>[3x]MRTGQQYLESLRDGRQVYVGGELIDDVTTHPKTSGYAKAIAEYYDLHLDPEHQDVLTFVDDDGVRKSMHWFLPRSKADAARRRAYHEFWFRHFQGGIFTRPPAGMHVVMYAQIDDPEPWGDNAVVAGGRTISFADNIRSQWQRVTTDDVALSPMFVDVQFDRGRDDALVETPMLSIVEQNDQGIVVRGWKAMGTSLPFVNELLVGNLWRPGQTSDQTVYAIVPVNTPGLSLVCRQSNATPDADPYDHPLSTIGDELDGMAYFDDVFIPWENVQHIGNPDHAKWYPQRQFDWVHIETQIRHAVHAELIVGLALLLTNALGTNNNPIVQSQLADLVRFRETCKAFAIAAEETGFTT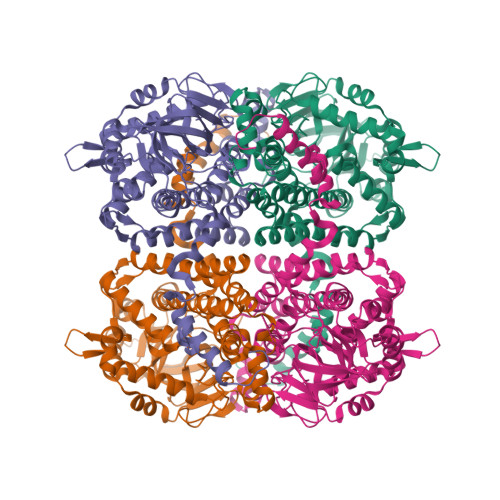AGGLFKPNNIYVDLGRAHYLENIHNAVNQLIEFCGRGVVMSPTKADFDHPFLGPKLEEALRGTSISARDRVSIFRQISERYLTQWGARHEMFEKFNGTPLYLVRLLTMQRTEYQVDGPLTDLARQVLGFGDTEALAARAAEVEKNSNWASVAYQPEYAREQDVRDGYYKETEKV Agrocinopine D-like  (C2-C2 linked; with two alpha-D-glucopyranoses) | C12 H23 O14 P | 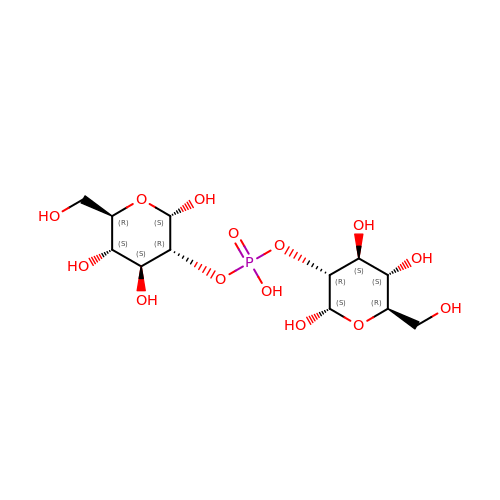DCDHSOINTWUWCZ-NCFXGAEVSA-N>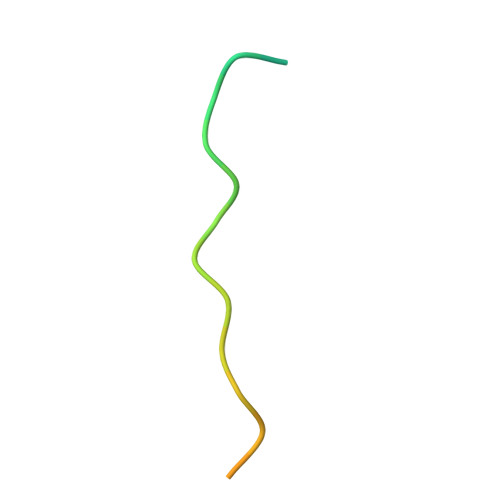 GSGVEDEDLSPRPSPNPHPVSQENLYFQ Peptide deformylases (PDFs) are metalloproteases that catalyze the removal of the formyl group from the initiator methionine, a critical step in the N-terminal methionine excision (NME) process. Most PDFs share a common catalytic core defined by three conserved sequence motifs (I, II, and III), which coordinate a metal ion and position key residues for substrate processing. All peptide-based PDF inhibitors share a common mechanism of action: they bind to the catalytic pocket of the enzyme, thereby preventing substrate access and inhibiting its deformylase activity. Furthermore, our investigation of V. cholerae, which encodes two type 1b PDFs with 50% sequence homology (Def1VCH and Def2VCH), demonstrated that both PDFs are catalytically active.

In contrast, the accessory PDF, Def2VCH, is encoded on chromosome 2 as a monocistronic unit. However, Def2VCH shows a specific pattern variation in the amino acids, described in E. coli, as responsible for ribosome binding. We found that Def2VCH specifically confers reduced susceptibility to the natural PDF inhibitor, ACT. To explore this possibility at the molecular level, we determined high-resolution crystal structures of both proteins in complex with ACT. In both structures, ACT binds in the same location within the catalytic pocket and adopts a nearly identical orientation and conformation, blocking access to the active site located at the bottom of a deep cavity in the protein core. In contrast, Def2VCH exhibited a different binding pattern. This is mainly due to the substitution of arginine 97 with a tyrosine, which weakens the interaction with ACT by abolishing important hydrogen bonds between the NH1 and NH2 atoms of Arg97 and solvent-exposed oxygen atoms of ACT (namely O20 and O27). Additionally, in the hydrophobic pocket containing the ACT P1' aliphatic chain, isoleucine at position 86 and leucine at position 125 in Def1VCH are substituted by glycine and phenylalanine, respectively, in Def2VCH. These substitutions likely contribute to the variation in ACT binding affinity between Def1VCH and Def2VCH, explaining their different capacities to confer resistance to this inhibitor. Conversely, substitution of tyrosine 97 with arginine in Def2VCH led to a marked reduction in the MIC, aligning with the resistance phenotype observed for Def1VCH.

>[2x]MHHHHHHGSGSGSAVLEILTAPDPRLRVQSKQVTDVASVQTLIDDLLDTLYATDNGIGLAAPQVGREEAIVVIDLSDNRDQPLVLINPKVVSGSNKEMGQEGCLSVPDYYADVERYTSVVVEALDREGKPLRIETSDFLAIVMQHEIDHLSGNLFIDYLSPLKQQMAMKKVKKHVKNRAR(2~{S})-3-(4-fluorophenyl)-2-[2-(3-hydroxyphenyl)ethanoylamino]-~{N}-[(1~{S})-1-phenylethyl]propanamide 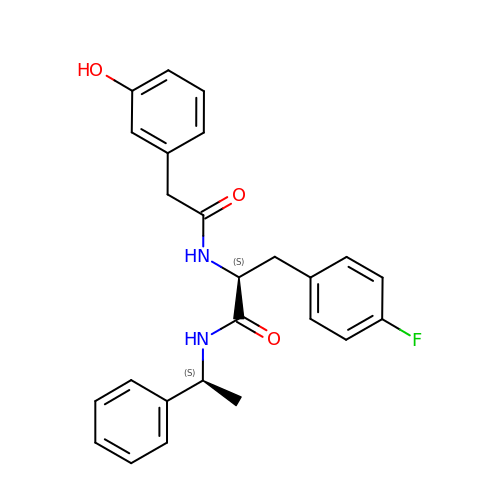| C25 H25 F N2 O3 | FYIWCUFRBHMEBW-SBUREZEXSA-N> VETGTIVRFNRP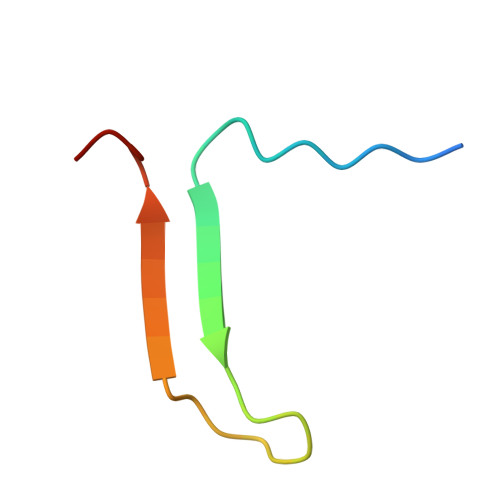FLMIIVPTDTQNIFFMSKVTNPKQA> HHHMTPEQREFLLEILAEI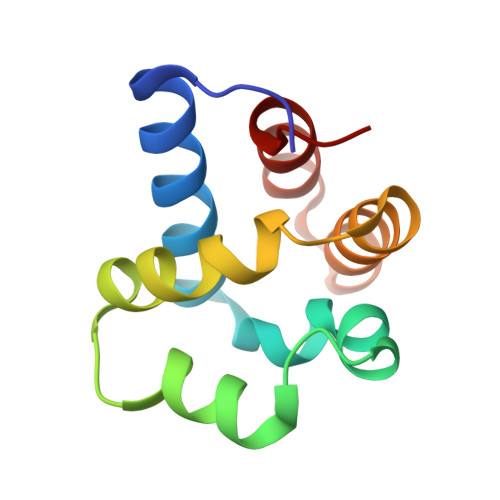IANLDPTKILEEPLRRGLLTPAELQEVLDLKTPEEQAKKLIDFILKLSPAEAQALIDALRAHGYQALADKLKKYLPLE> MAREFKRSDRVAQEIQKEIAVILQREVKDPRIGMVTVSDVEVSSDLSYAKIFVTFLFDHDEMAIEQGMKGLEKASPYIRSLLGKAMRLRIVPEIRFIYDQSLVEGMR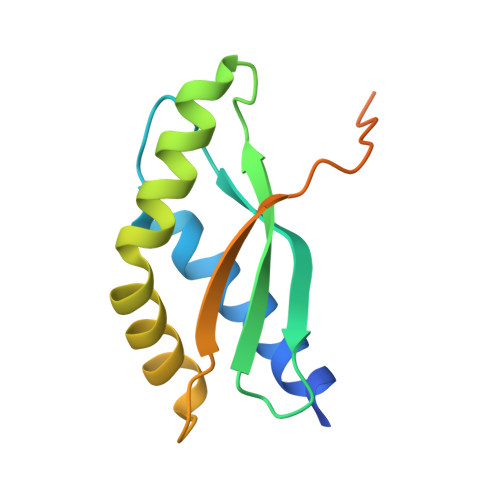MSNLVTNVVREDEKKHVEESN>GSMAVEVEVPTQVPAHIGIIMDGNGRWAKKRMQPRVFGHKAGMEALQTVTKAANKLGVKVITVYAFSTENWTRPDQEVKFIMNLPVEFYDNYVPELHANNVKIQMIGETDRLPKQTFEALTKAEELTKNNTGL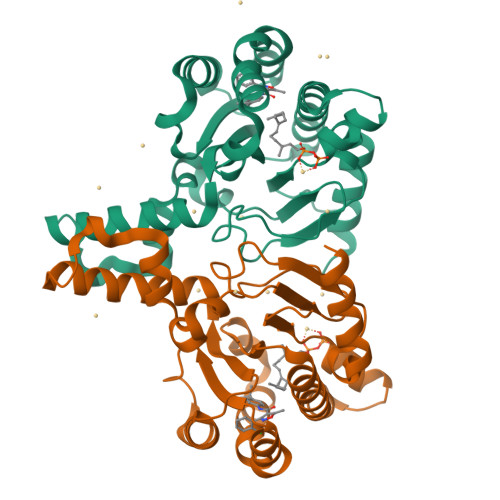ILNFALNYGGRAEITQALKLISQDVLDAKINPGDITEELIGNYLFTQHLPKDLRDPDLIIRTSGELRLSNFLPWQGAYSELYFTDTLWPDFDEAALQEAILAYNRRHRRFGGV[2x]>[2x]MEEPEEPADSGQSLVPVYIYSPEYVSMCDSLAKIPKRASMVHSLIEAYALHKQMRIVKPKVASME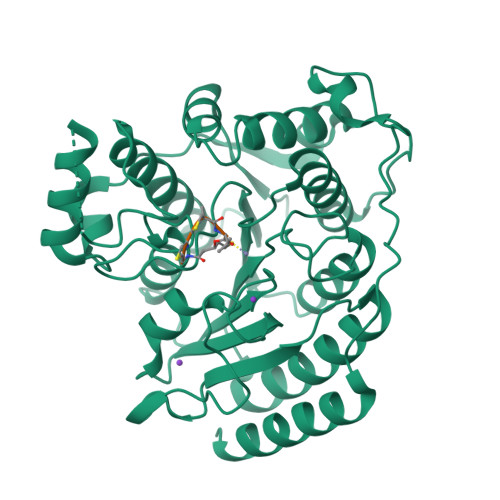EMATFHTDAYLQHLQKVSQEGDDDHPDSIEYGLGYDCPATEGIFDYAAAIGGATITAAQCLIDGMCKVAINWSGGWHHAKKDEASGFCYLNDAVLGILRLRRKFERILYVDLDLHHGDGVEDAFSFTSKVMTVSLHKFSPGFFPGTGDVSDVGLGKGRYYSVNVPIQDGIQDEKYYQICESVLKEVYQAFNPKAVVLQLGADTIAGDPMCSFNMTPVGIGKCLKYILQWQLATLILGGGGYNLANTARCWTYLTGVILGKTLSSEIPDHEFFTAYGPDYVLEITPSCRPDRNEPHRIQQILNYIKGNLKHVVIEGRGSHHHHHH;>XGCCV[2x]The Drosophila melanogaster Serpin 42 Da gene (previously Serpin 4) encodes a serine protease inhibitor that is capable of remarkable functional diversity through the alternative splicing of four different reactive centre loop exons. Eight protein isoforms of Serpin 42 Da have been identified to date, targeting the protease inhibitor to both different proteases and cellular locations. Spn42Da is in the highly stable ‘cleaved’ conformation, with the cleaved RCL inserted into β-sheet A to form the 4th strand in the six stranded central β-sheet. Spn42Da has a typical serpin fold comprising a mixed α-β secondary structure with an N-terminal helical region and a C-terminal β-barrel fold.

The first crystal form, designated Spn42Da-1, crystallised in the C2221 spacegroup (a = 59.74 Å, b = 125.95 Å, c = 119.94 Å) and diffracted to a resolution of 1.7 Å. The structures are of high quality; the Spn42Da-1 structure refined to a Rwork/Rfree of 16.51% and 18.81% respectively, and the Spn42Da-2 structure to a Rwork/Rfree of 16.58% and 18.54% respectively. Within the Ramachandran plot, the Spn42Da-1 structure contains 98.9% of residues in the favoured region and no residues in the outlier regions. The Spn42Da-1 structure scored in the 100th percentile of structures in MolProbity, with a clashscore of 2.39 for all atoms and an overall MolProbity score of 1.02. Spn42Da-1 has 369 amino acids from residue number 4 to 387 of the molecule, with three loops (D86-Q88, D191-R194, K367) and seven residues of the RCL (A343-E349) missing due to poor electron density - most likely reflecting protein cleavage or their mobility within the protein. In the Spn42Da-1 crystal structure, clear electron density ends after the P1 Arg residue, suggesting that the RCL was cleaved after this consensus recognition site between the P1 Arg and the P1’ Ala residues. As such, except for the presence of an extra six C-terminal amino acids within the Spn42Da-1 structure there are no major regions of difference between the two crystal forms. The two crystal forms of Spn42Da are structurally homologous with no large conformational differences and an RMSD of 0.35 Å across 363 aligned residues. The last four residues of the Spn42Da protein, corresponding to a likely ER retention signal, are not present in the density of either structure.

> MMADAAHQEFARRLALFSINVYGKLSGQKPGENIVFSPFSIQTCAAMARLGAENETATQLDQGLGLASSDPEQIAHSFHQVLAAYQDSQILRIANKIFVMDGYQLRQEFDQLLSKQFLSAAQSVDFSKNVQAAATINNWVEQRTNHLIKDLVPADVLNSESRLVLVNAIHFKGTWQHQFAKHLTRPDTFHLDGERTVQVPMMSLKERFRYADLPALDAMALELPYKDSDLSMLIVLPNTKTGLPALEEKLRLTTLSQITQSLYETKVALKLPRFKAEFQVELSEVFQKLGMSRMFSDQAEFGKMLQSPEPLKVSAIIHKAFIEVNEEGTEAAAATGMAVRRKRAIMSPEEPIEFFADHPFTYVLVHQKDLPLFWGSVVRLEENTFASSEHDEL> ERTINLYPLTNYTFGTKEPLYEKDSSVAARFQRMREEFDKIGMRRTVEGVLIVHEHRLPHVL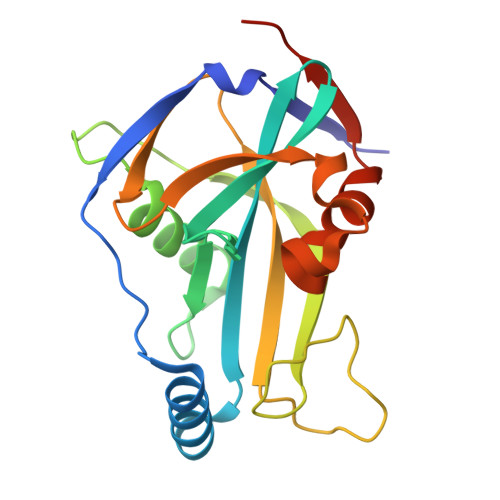LLQLGTTFFKLPGGELNPGEDEVEGLKRLMTEILGRQDGVLQDWVIDDCIGNWWRPNFEPPQYPYIPAHITKPKEHKKLFLVQLQEKALFAVPKNYKLVAAPLFELYDNAPGYGPIISSLPQLLSRFNFIYNLEHHHHHH>SHMDPVSVWGNTPLATVDPEIHDLIEKEKRRQCRGIELIASENFTSFAVIEALGSALTNKYSEGMPGNRYYGGNEYIDQIENLCRSRALQAFHLDAQSWGVNVQPYSGSPANFAAYTAVLNPHDRIMGLDLRSGGHLTHGYYTSGGKKISATSIYFESLPYKVNSTTGYIDYDRLEEKALDFRPKLIICGGSAYPRDWDYKRFREVADKCGALLLCDMAHTSGLVAAQEVNSPFEYCDIVTTTTHKSLRGPRAGMIFYRKGPKPPKKGQPENAVYDFEDKINFAVFPSLQGGPHNHQIGALAVALKQAASPGFKAYAKQVKANAVALGKYLMGKGYSLVTGGTENHLVLWDLRPLGLTGYKVEKLCDLCNITVNKN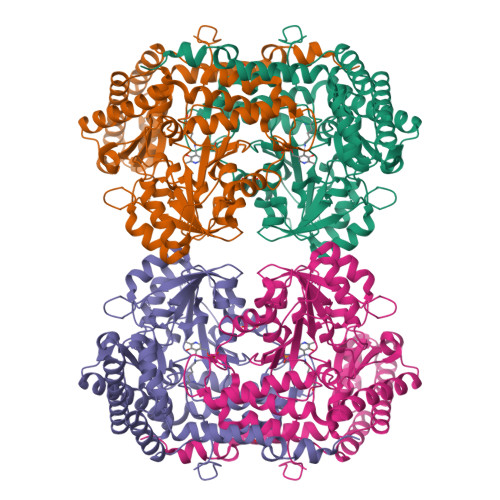AVFGDSSALAPGGVRIGAPAMTSRGLVEKDFEQIGEFLHRAVTLTLEIQKEHGKLLKDFNKGLVNNKAIEDLKADVEKFSALFDMPGFLVSEMKYKD[2x]> MAKHLFTSESVSEGHPDKIADQISDAVLDAI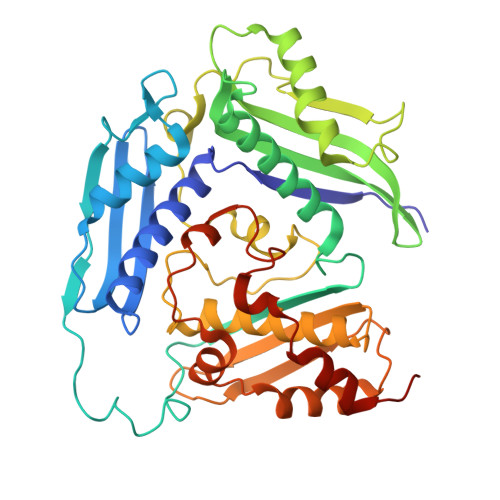LEQDPKARVACETYVKTGMVLVGGEITTSAWVDIEEITRNTVREIGYVHSDMGFDANSCAVLSAIGKQSPDINQGVDRADPLEQGAGDQGLMFGYATNETDVLMPAPITYAHRLVQRQAEVRKNGTLPWLRPDAKSQVTFQYDDGKIVGIDAVVLSTQHSEEIDQKSLQEAVMEEIIKPILPAEWLTSATKFFINPTGRFVIGGPMGDCGLTGRKIIVDTYGGMARHGGGAFSGKDPSKVDRSAAYAARYVAKNIVAAGLADRCEIQVSYAIGVAEPTSIMVETFGTEKVPSEQLTLLVREFFDLRPYGLIQMLDLLHPIYKETAAYGHFGREHFPWEKTDKAQLLRDAAGLKHHHHHH> MPLDAGGQNSTQMVLAPGASIFRCRQCGQTISRRDWLLPMGGDHEHVVFNPHGYIHRVWCFSLAQGLNLIGRPSGEFSWFKGYDWTVAQCGQCGSHLGWHYEGGSQPQTFFGLI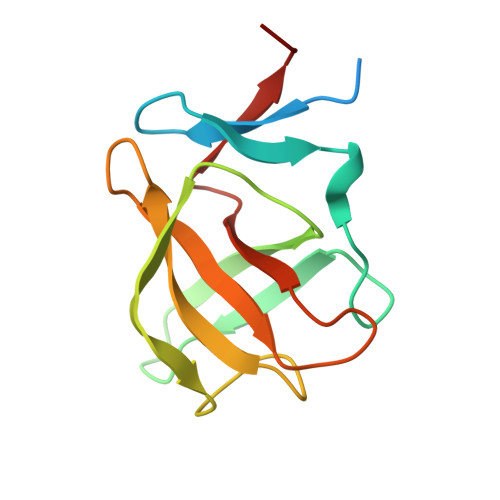KDRLAEGPAD>[3x]MDYKDDDDKLEATMAMSSKISVELQRVAALPAQGCSNTGFQNDEDGFENQNPSGNDHSLRNRVVQNREHENGKQVEEHITIGQDSLRKDEEEEDDQETHRKGCLERMCGRMSDFCREHKTTLRYIIWGILIAGYLALVIAACVMNFHRALPLFVITVVAIFFVVWDHLMAKYESQIARFLSPGQRLLDSHWFWLKWVIWGCLILGVILWLVFDTAKLGQQQLVSFGGLIIYTSLTFLFSKHPTKVYWR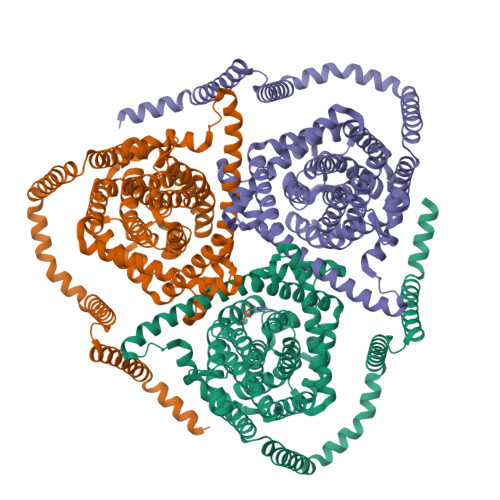PVFWGIGLQFLLGLLILRTEPGFMAFDWLGKQVQTFLGYSDAGASFVFGEKYTDHFFAFKVLPIVIFFSTVMSMLYYLGLMQWIIRKVGWVMLVTMGTSPVESVVASGNIFIGQTESPLLVRPYLPYVTKSELHAIMTAGFSTIAGSVLGAYISFGVSSSHLLTASVMSAPAALAISKLFWPETETPKINLKNAMKMESGDSRNLLEAATQGASSSISLVANIAVNLIAFLALLSFMNSALSWLGNMFDYPQLSFEVICSYVFMPFAFMMGVDWQDSFMVAKLIGYKTFFNEFVAYQQLSKLISLRQVGGPKFVDGVQQYMSMRSEAISTYALCGFANFGSLGIVIGGLTSMAPSRKRDITAGAMRALIAGTIACFLTACIAGMLTNTPVDINCHHILENAFNSGLVRNTTNVVSCCQGLLSSAVVKGPGEVIPTGNHSLYSLKNCCNLLNTPTLNCSWIPNVLSNS> RICEVWACNLDEEMKKIRQVIRKYNYVAMDTEFPGVVARPIGEFRSNADYQYQLLRCNVDLLKIIQLGLTFMNEQGEYPPGTSTWQFNFKFNLTEDMYAQDSIELLTTSGIQFKKHEEEGIETQYFAELLMTSGVVLCEGVKWLSFHSGYDFGYL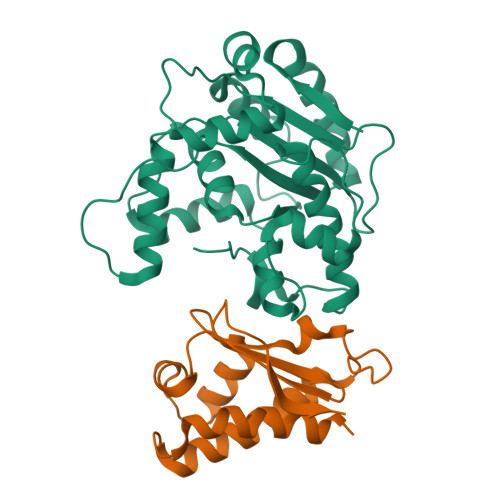IKILTNSNLPEEELDFFEILRLFFPVIYDVKYLMKSCKNLKGGLQEVAEQLELERIGPQHQAGSDSLLTGMAFFKMREMFFEDHIDDAKYCGHLYGL;> HMQLEIQVALNFIISYLYNKLPRRRVNIFGEELERLLKKKYEGHWYPEKPYKGSGFRCIHIGEKVDPVIEQASKESGLDIDDVRGNLPQDLSVWIDPFEVSYQIGEKGPVKVLYVD>MAGRWLDPLWAPGFLCVALILETASGAGDLSTKAHGHIQFSARGVNQTAMADCRAVCSLNTSDRCDFVKRNPDCHSEGGYLDYLKGIFCYFPPNLLPLAITLYVFWLLYLFLILGVTAAKFFCPNLSAISTSLKLSHNVAGVTFLAFGNGAPDIFSALVAFSDPRTAGLAIGALFGAGVLVTTVVAGGITILRPFMAASRPFLRDITFYMVAVFLTFTALYLGRITLVWALGYLGLYVFYVVTVIICTWVYQRQRSRSLVHSISETPELLTDSEEDQMSSNTNSYDYGEEYRPLLLGEETTGQILLQALNPLDYRKWRTQSISCKLLKVAKLPVEFLLLLTVPVVDPDKDDRNWKRPLNCLQLVISPLVLVLTLQSGVYGIYEIGGLLPVWAVVVIVGTALASVTFFATSNSEPPRLHWLFAFLGFLTSALWINAAATEVVNILRSLGVVFRLSNTVLGLTLLAWGNSIGDAFSDFTLARQGYPRMAFSACFGGIIFNILVGVGLGCLLQIVRSHASEVKLEPDGLLVWVLASALGLSLVFSLVSVPLQCFQLSKAYGLCLLLFYICFIVVVLLTEFGVIHLKAD[3x]

As a key mitochondrial Ca2+ transporter, NCLX regulates intracellular Ca2+ signalling and vital mitochondrial processes. Here we report the cryogenic electron microscopy (cryo-EM) structures of rat NCLX in cytosol-facing (intermembrane space) and matrix-facing conformations, with and without Ca2+. Each NCLX protomer contains twelve transmembrane helices and two sets of helical hairpins/bundles roughly parallel to the membrane. The structure comprises a transport domain, which mediates NCLX trimer formation at the centre, and a gate domain, located on the periphery without contacting other protomers.

We selected rat NCLX (83% sequence identity with human NCLX) for cryo-EM due to its favourable biochemical behaviour. Cryo-EM studies on NCLX under Ca2+-bound (2 mM Ca2+, pH 7.4) or Ca2+-free (5 mM ethylene glycol tetraacetic acid (EGTA), without adding Ca2+, pH 5.5 and 7.4) conditions produced maps with resolutions of up to 2.15 Å, enabling unambiguous modelling of NCLX. Under Ca2+-free conditions, we also observed distinct assemblies, including all three protomers in matrix-facing; one or two in cytosol-facing; or all three in cytosol-facing conformation. Our structure determined at a low pH of 5.5 without Ca2+ presumably represents proton-loaded NCLX, given the ~100-fold higher proton concentration compared with the transporter’s typical operating conditions. Notably, under this condition, the structure exhibits cytosol-open conformations across all protomers within a trimer, suggesting that this conformation is predominant at low pH. By contrast, the structure determined at pH 7.4 without Ca2+ displays a combination of cytosol- and matrix-open, or all matrix-open, conformations within a trimer, compatible with NCLX potentially in mixed protonated states. This pH-dependent shift in conformational state distribution aligns with our finding that NCLX operates a H+-coupled transport process. Furthermore, we found that, for each protomer, the overall structure of this putative proton-bound NCLX is similar to the Ca2+-bound form, with the N-terminal half of TM2 rotating around the Ca2+-binding site along the interface with the gate domain. This rotation is presumably caused by local changes in the Ca2+-binding site configuration, whereas the domain-interface residues of TM2 remain staying on the interface.>[4x]MGSSHHHHHHGENLYFQSTKKSAAEASKKPRQKRTATKAYNVTQAF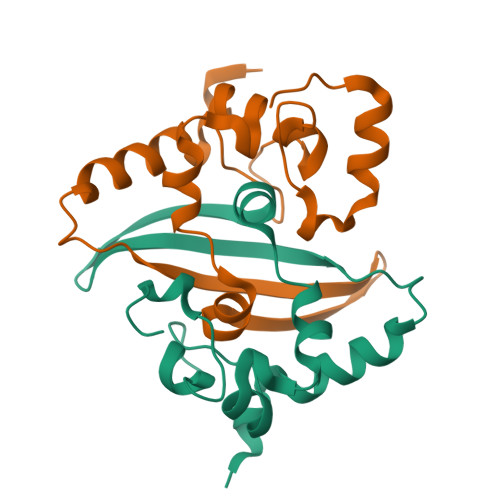GRRGPEQTQGNFGDQELIRQGTDYKHWPQIAQFAPSASAFFGMSRIGMEVTPSGTWLTYTGAIKLDDKDPNFKDQVILLNKHIDAYKTFP>GAMEDLIPLVNRLQDAFSAIGQNADLDLPQIAVVGGQSAGKSSVLENFVGRDFLPRGSGIVTRRPLVLQLVNATTEYAEFLHSKGKKFTDFEEVRLEIEAETDRVTGTNKGISPVPINLRVYSPHVLNLTLVDLPGMTHVPVGDQPPDIEFQIRDMLMQFVTKENCLILAVSPANSDLAHSDALKVAKEVDPQGQRTIGVITKLDLMDEGTDARDVLENKLLPLRRGYIGVVNRSQKDI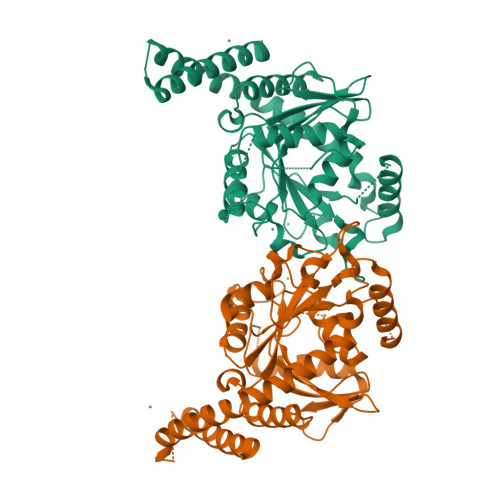DGKKDITAALAAERKFFLSHPSYRHLADRMGTPYLQKVLNQQLTNHIRDTLPGLRNKLQSQLLSIEKEVEEYKNFRPDDPNTLMEESAEQAQRRDEMLRMYHALKEALSIIGDIN[2x]>NLGLDCDEHSSESRCCRYPLTVDFEAFGWDWIIAPKRYKANYCSGQCEYMFMQKYPHTHLVQQANPRG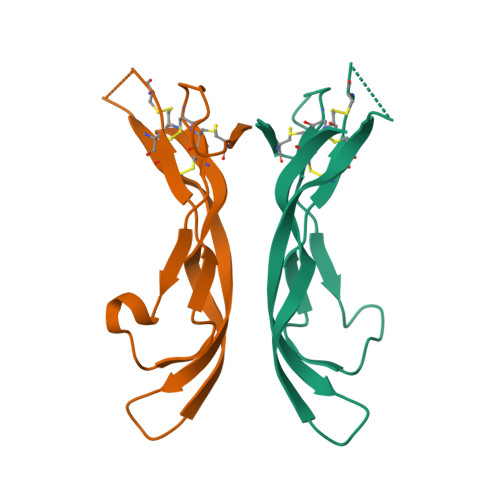SAGPCCTPTKMSPINMLYFNDKQQIIYGKIPGMVVDRCGCS[2x]Here we report the discovery of type IV borosin natural product pathways (termed ‘split borosins’), featuring an iteratively acting α-N-methyltransferase and separate precursor peptide substrate from the metal-respiring bacterium Shewanella oneidensis. The α-N-methyltransferase SonM from Shewanella oneidensis MR-1 iteratively methylates its substrate SonA at two residues, SonA-L63 and SonA-I65, in an N-to-C terminal fashion on the core peptide. Complexes of SonM and SonA form dimers of heterodimers. A five helical bundle at the N-terminus of SonA, now referred to as the borosin binding domain (BBD; 1–53), serves as the SonA leader peptide and is homologous to a portion of the fused clasp region of OphMA.

While we were unable to obtain crystals of SonM or SonA individually, we were successful in determining a series of structures of SonM in complex with SonA, either bound or unbound with the methyl-donating cofactor S-adenosylmethionine (SAM) or its product S-adenosylhomocysteine (SAH). While SAH is bound to the protein by an extensive network of interactions, the apo structure reveals the presence of water molecules filling the cofactor’s cavity. Most differences between the structures relate to concerted rotamer changes due to steric hindrance upon SAH binding. Specifically, upon SAH binding, the side chain of SonM-Y93 relocates by 1 Å and the side chain of SonM-I234 rotates nearly 180° to increase the cofactor binding pocket volume. Interestingly, changes in SonM-Y93 conformation induces a conformation change (up to 1.8 Å) of the side chain of i−2 SonA-MLE63. These changes appear necessary to sterically allow for cofactor exchange. We therefore find that SonM can adopt a closed conformation in the absence of the core peptide and with cofactor (SAM) bound, and also in the absence of cofactor with the core peptide bound.

>MGSLVCVGTGLQLAGQISVLSRSYIEHADIVFSLLPDGFSQRWLTKLNPNVINLQQFYAQNGEVKNRRDTYEQMVNAILDAVRAGKKTVCALYGHPGVFACVSHMAITRAKAEGFSAKMEPGISAEACLWADLGIDPGNSGHQSFEASQFMFFNHVPDPTTHLLLWQIAIAGEHTLTQFHTSSDRLQILVEQLNQWYPLDHEVVIYEAANLPIQAPRIERLPLANLPQAHLMPISTLLIPPAKKLEYNYAILAKLGIGPEDLG[2x];>[2x]MSGLSDFFTQLGQDAQLMEDYKQNPEAVMRAHGLTDEQINAVMTGDMEKLKTLSGDSSYQSYLVISHGNGD>SNAMTDDKKIRAAIVGYGNIGRYALQALREAPDFEIAGIVRRNPAEVPFELQPFRVVSDIEQLESVDVALVCSPSREVERTALEILKKGICTADSFDIHDGILALRRSLGDAAGKSGAAAVIASGWDPGSDSVVRTLMQAIVPKGITYTNFGPGMSMGHTVAVKAIDGVKAALSMTIPLGTGVHRRMVYVELLPGHNLEEVSAAIKADEYFVHDETHVIQVDEVDALIDMGHGVRMVRKGVSGSTQNQRMSFDMEINNPALTGQVLVCAARAAMRQQPGAYTLQEIPVID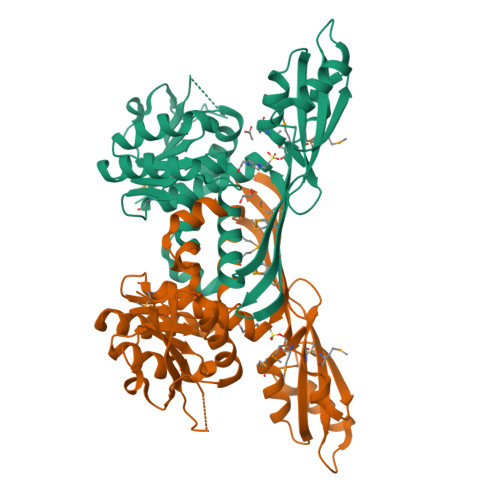LLPGDREQWIGKLC[2x]>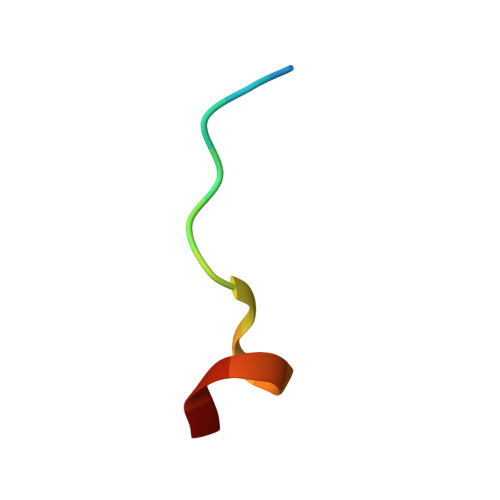 XTPEAPPCYMDVIX Human alpha-2 macroglobulin-like 1 (A2ML1) is a monomeric member of the A2M superfamily (A2MF) of protease inhibitors and complement factors. The functional inhibitory unit of A2ML1 is a monomer that depends on covalent binding of the protease (mediated by A2ML1’s thioester) to achieve inhibition. A2MF protease inhibitors utilize a unique trapping mechanism that pseudo-inhibits proteases regardless of their catalytic class. Trapped proteases remain catalytically active but are prevented from cleaving protein substrates through steric hindrance imposed by the inhibitor following a proteolytically triggered conformational change.

Structures of native A2ML1 were determined by X-ray crystallography and cryo-EM at resolutions of 4.4 and 3.1 Å, respectively. Overall, the cryo-EM and X-ray structures are very similar with an overall root mean square deviation (RMSD) of 2.0 Å for the entire molecule. Native A2ML1 is organized in two structural units connected by the MG7 domain. The N-terminal residues Glu19-Phe787 constitute the MG-ring formed by MG domains 1–6, the associated LNK region, and the bait region. The C-terminal domains CUB, TE, and MG8 encompassing residues His904-Glu1454 form a compact structure with extensive CUB-TE and TE-MG8 interactions, which we call the CTM8 body. In both the EM and the X-ray structures of native A2ML1, it is not possible to model residues His696-Asp726, suggesting substantial flexibility of the intact bait region in accordance with its accessibility toward proteases. However, in both structures, it is evident that the strictly conserved residues Arg730-Pro734 pass through the same narrow opening that houses the Nt-α′ in complement A2MF proteins. In particular, Tyr732 and Phe733 in the BR-C region form a hydrophobic plug inserted between the highly conserved Leu130, Leu216, and Val598. In native A2ML1, the bait region is threaded through a hydrophobic channel, suggesting that disruption of this arrangement by bait region cleavage triggers the extensive conformational changes that result in protease inhibition.

> ELPNYLVTLPARLNFPSVQKVCLDLSPGYSDVKFTVTLETKDKTQKLLEYSGLKKRHLHCISFLVPPPAGGTEEVATIRVSGVGNNISFEEKKKVLIQRQGNGTFVQTDKPLYTPGQQVYFRIVTMDSNFVPVNDKYSMVELQDPNSNRIAQWLEVVPEQGIVDLSFQLAPEAMLGTYTVAVAEGKTFGTFSVEEYVLPKFKVEVVEPKELSTVQESFLVKICCRYTYGKPMLGAVQVSVCQKANTYWYREVEREQLPDKCRNLSGQTDKTGCFSAPVDMATFDLIGYAYSHQINIVATVVEEGTGVEANATQNIYISPQMGSMTFEDTSNFYHPNFPFSGKIRVRGHDDSFLKNHLVFLVIYGTNGTFNQTLVTDNNGLAPFTLETSGWNGTDVSLEGKFQMEDLVYNPEQVPRYYQNAYLHLRPFYSTTRSFLGIHRLNGPLKCGQPQEVLVDYYIDPADASPDQEISFSYYLIGKGSLVMEGQKHLNSKKKGLKASFSLSLTFTSRLAPDPSLVIYAIFPSGGVVADKIQFSVEMCFDNQVSLGFSPSQQLPGAEVELQLQAAPGSLCALRAVDESVLLLRPDRELSNRSVYGMFPFWYGHYPYQVAEYDQCPVSGPWDFPQPLIDPMPQGHSSQRSIIWRPSFSEGTDLFSFFRDVGLKILSNAKIKKPVDCSHRSPEYSTAMGAGGGHPEAFESSTPLHQAEDSQVRQYFPETWLWDLFPIGNSGKEAVHVTVPDAITEWKAMSFCTSQSRGFGLSPTVGLTAFKPFFVDLTLPYSVVRGESFRLTATIFNYLKDCIRVQTDLAKSHEYQLESWADSQTSSCLCADDAKTHHWNITAVKLGHINFTISTKILDSNEPCGGQKGFVPQKGRSDTLIKPVLVKPEGVLVEKTHSSLLCPKGKVASESVSLELPVDIVPDSTKAYVTVLGDIMGTALQNLDGLVQMPSGCGEQNMVLFAPIIYVLQYLEKAGLLTEEIRSRAVGFLEIGYQKELMYKHSNGSYSAFGERDGNGNTWLTAFVTKCFGQAQKFIFIDPKNIQDALKWMAGNQLPSGCYANVGNLLHTAMKGGVDDEVSLTAYVTAALLEMGKDVDDPMVSQGLRCLKNSATSTTNLYTQALLAYIFSLAGEMDIRNILLKQLDQQAIISGESIYWSQKPTPSSNASPWSEPAAVDVELTAYALLAQLTKPSLTQKEIAKATSIVAWLAKQHNAYGGFSSTQDTVVALQALAKYATTAYMPSEEINLVVKSTENFQRTFNIQSVNRLVFQQDTLPNVPGMYTLEASGQGCVYVQTVLRYNILPPTNMKTFSLSVEIGKARCEQPTSPRSLTLTIHTSYVGSRSSSNMAIVEVKMLSGFSPMEGTNQLLLQQPLVKKVEFGTDTLNIYLDELIKNTQTYTFTISQSVLVTNLKPATIKVYDYYLPDEQATIQYSDPCE> RSEYVAPRSVWEARLAQVWEQVLNVPQVGALDDFFALGGHSLRAMRVLSSMHNEYQVDIPLRILFEKPTIQELAAFIEETAKGNVFSIEPVQKQAYYPVSSAQKRMYILDQFEGVGISYNMPSTMLIEGKLERTRVEAAFQRLIARHESLRTSFAVVNGEPVQNIHEDVPFALAYSEVTEEEARELVSSLVQPFDLEVAPLIRVSLLKIGEDRYVLFTDMHHSISDGVSSGILLAEWVQLYQGDVLPELRIQYKDFAVWQQEFSQSAAFHKQEAYWLQTFADDIPVLNLPTDFTRPSTQSFAGDQCTIGAGKALTEGLHQLAQATGTTLYMVLLAAYNVLLAKYAGQEDIIVGTPITGRSHADLEPIVGMFVNTLAMRNKPQREKTFSEFLQEVKQNALDAYGHQDYPFEELVEKLAIARDLSRNPLFDTVFTFQNSTEEVMTLPECTLAPFMTD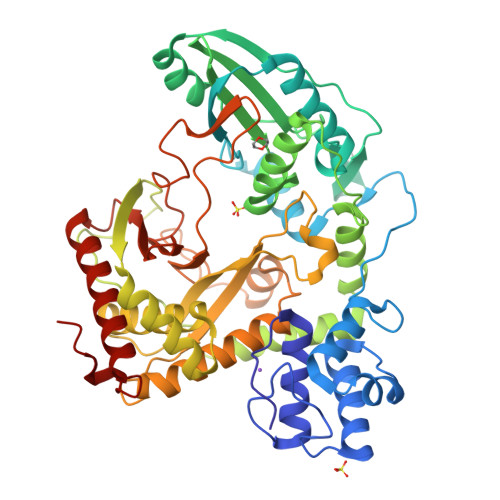ETGQHAKFDLTFSATEEREEMTIGVEYSTSLFTRETMERFSRHFLTIAASIVQNPHIRLGEIDML>SNKCDVVVVGGGISGMAAAKLLHDSGLNVVVLEARDRVGGRTYTLRNQKVKYVDLGGSYVGPTQNRILRLAKELGLETYKVNEVERLIHHVKGKSYPFRGPFPPVWNPITYLDHNNFWRTMDDMGREIPSDAPWKAPLAEEWDNMTMKELLDKLCWTESAKQLATLFVNLCVTAETHEVSALWFLWYVKQCGGTTRIISTTNGGQERKFVGGSGQVSERIMDLLGDRVKLERPVIYIDQTRENVLVETLNHEMYEAKYVISA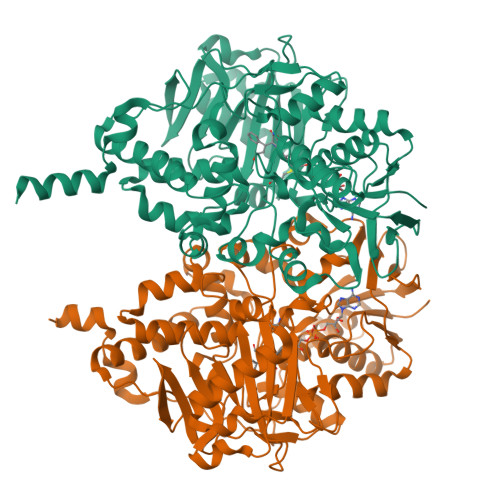IPPTLGMKIHFNPPLPMMRNQMITRVPLGSVIKCIVYYKEPFWRKKDYCGTMIIDGEEAPVAYTLDDTKPEGNYAAIMGFILAHKARKLARLTKEERLKKLCELYAKVLGSLEALEPVHYEEKNWCEEQYSGGCYTTYFPPGILTQYGRVLRQPVDRIYFAGTETATHWSGYMEGAVEAGERAAREILHAMGKIPEDEIWQSEPESVDVPAQPITTTFLERHLPSVPGLLRLIGLTTIFSATALGFLAHKRGLLVRV[2x]>AENDKPQYLSDWWHQSVNVVGSYHTRFGPQIRNDTYLEYEAFAKKDWFDFYGYADAPVFFGGNSDAKGIWNHGSPLFMEIEPRFSIDKLTNTDLSFGPFKEWYFANNYIYDMGRNKDGRQSTWYMGLGTDIDTGLPMSLSMNVYAKYQWQNYGAANENEWDGYRFKIKYFVPITDLWGGQLSYIGFTNFDWGSDLGDDSGNAINGIKTRTNNSIASSHILALNYDHWHYSVVARYWHDGGQWNDDA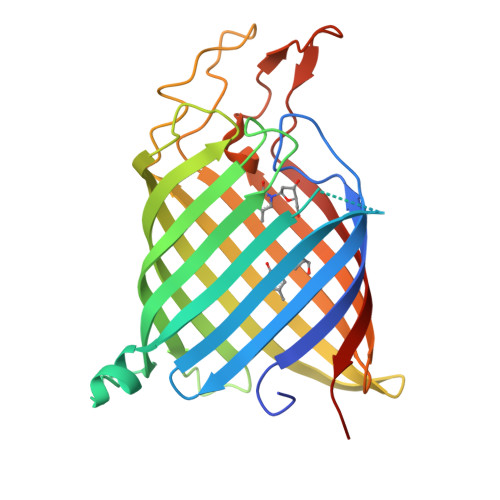ELNFGNGNFNVRSTGWGGYLVVGYNFHHHHHH[2x]> GLVPRGSHMSGATEACLPAGQRKSGMNINFYQYSLKDSSTYSNAAYMAYGYASKTKLGSVGGQTDISIDYNIPCVSSSGTFPCPQEDSYGNWGCKGMGACSNSQGIAYWSTDLFGFYTTPTNVTLEMTGYFLPPQTGSYTFSFATVDDSAILSVGGSIAFECCAQEQPPITSTNFTINGIKPWDGSLPDNITGTVYMYAGYYYPLKVV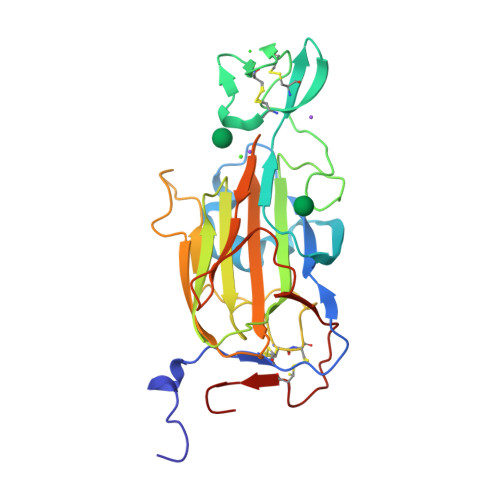YSNAVSWGTLPISVELPDGTTVSDNFEGYVYSFDDDLSQSNCTIPDPSIH>MVERYSLSPMKDLWTEEAKYRRWLEVELAVTRAYEELGMIPKGVTERIRNNAKIDVELFKKIEEKTNHDVVAFVEGIGSMIGEDSRF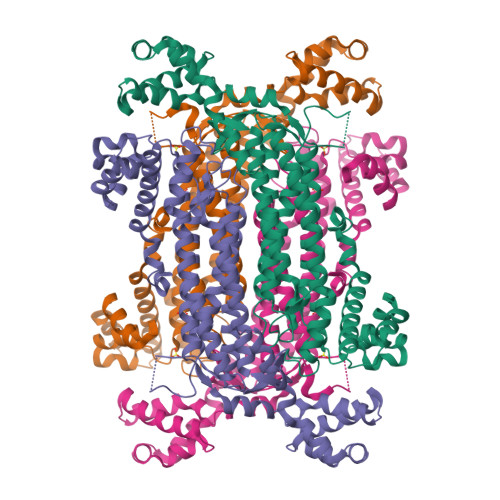FHYGLTSSDVLDTANSLALVEAGKILLESLKEFCDVLWEVANRYKHTPTIGRTHGVHAEPTSFGLKVLGWYSEMKRNVQRLERAIEEVSYGKISGAVGNYANVPPEVEEKALSYLGLKPEPVSTQVVPRDRHAFYLSTLAIVAAGIERIAVEIRHLQRTEVLEVEEPFRKGQRGSSAMPHKKNPITCERLTGLSRMMRAYVDPSLENIALWHERDISHSSVERYVFPDATQTLYYMIVTATNVVRNMKVNEERMKKNIDLTKGLVFSQRVLLKLIEKGLTRKEAYDIVQRNALKTWNSEKHFLEYLLEDEEVKKLVTKEELEELFDISYYLKHVDHIFERFEKE[2x]>MSQHNEKNPHQHQSPLHDSSEAKPGMDSLAPEDGSHRPAAEPTPPGAQPTAPGSLKAPDTRNEKLNSLEDVRKGSENYALTTNQGVRIADDQNSLRAGSRGPTLLEDFILREKITHFDHERIPERIVHARGSAAHGYFQPYKSLSDITKADFLSDPNKITPVFVRFSTVQGGAGSADTVRDIRGFATKFYTEEGIFDLVGNNTPIFFIQDAHKFPDFVHAVKPEPHWAIPQGQSAHDTFWDYVSLQPETLHNVMWAMSDRGIPRSYRTMEGFGIHTFRLINAEGKATFVRFHWKPLAGKASLVWDEAQKLTGRDPDFHRRELWEAIEAGDFPEYELGFQLIPEEDEFKFDFDLLDPTKLIPEELVPVQRVGKMVLNRNPDNFFAENEQAAFHPGHIVPGLDFTNDPLLQGRLFSYTDTQISRLGGPNFHEIPINRPTCPYHNFQRDGMHRMGIDTNPANYEPNSINDNWPRETPPGPKRGGFESYQERVEGNKVRERSPSFGEYYSHPRLFWLSQTPFEQRHIVDGFSFDLSKVVRPYIRERVVDQLAHIDLTLAQAVAKNLGIELTDDQLNITPPPDVNGLKKDPSLSLYAIPDGDVKGRVVAILLNDEVRSADLLAILKALKAKGVHAKLLYSRMGEVTADDGTVLPIAATFAGAPSLTVDAVIVPCGNIADIADNGDANYYLMEAYKHLKPIALAGDARKFKATIKIADQGEEGIVEADSADGSFMDELLTLMAAHRV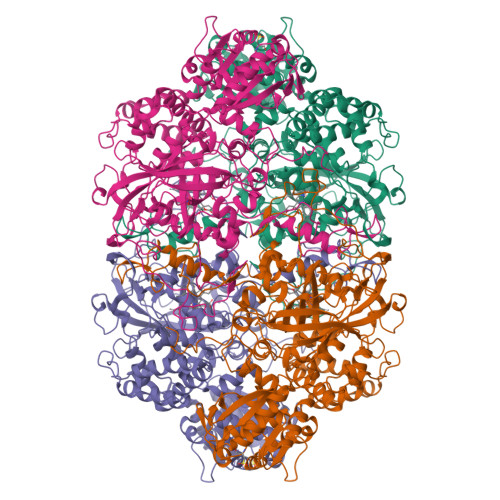WSRIPKIDKIPA[4x]>AAGGLDDANKFNYTGLGGPLNWYGLDEANEACAKGKHQSPIVIDSAAIDYAASGSLKLDLPLADGSKLENLGFGLQVTLTNGSLTANSKTYTLAQFHFHTPSEHHVNEEHFPMEVHFVFQTAAKETAVVGFFFQLSEVGDSVPLFDSVFAPIDNIPDAGTSTTTGQLDFGGLLDHFNR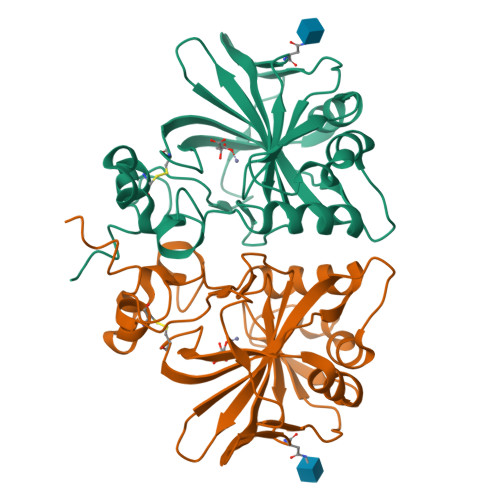HGVYQYTGSLTTPPCTEEVMWNLSTEPLPLTVQGYNKVKKIIKYNARYTQNALGQDNLLEVAAQKL[2x]> MAKGKQIPLTFDTYQDASTGAQVTRLTPPDVTCHRNYFYQKCFTRDGSKLLFGGAFDGPWNYYLLDLNTQVATQLTEGRGDNTFGGFLSPDDDALFYVKDGRNLMRVDLATLEENVVYQVPAEWVGYGTWVANSDCTKLVGIEIRREDWVPLTDWKKFHEFYFTKPCCRLMRVDLKTGESTVILQENQWLGHPIYRPYDDSTVAFCHEGPHDLVDARMWLINEDGTNMRKVKTHAEGESCTHEFWVPDGSALVYVSYLKGSPDRFIYSADPETLENRQLTSMPACSHLMSNYDGSLMVGDGSDAPVDVQDDSGYKIENDPFLYVFNMKNGTQHRVARHDTSWKVFEGDRQVTHPHPSFTPDDKQ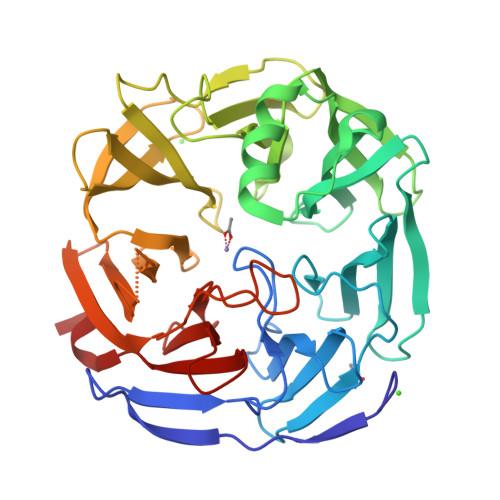ILFTSDVHGKPALYLATLPESVWK~{N}-[4-(6,7-dimethoxyquinazolin-4-yl)oxyphenyl]-2-(1-ethylpyrazol-4-yl)ethanamide | C23 H23 N5 O4 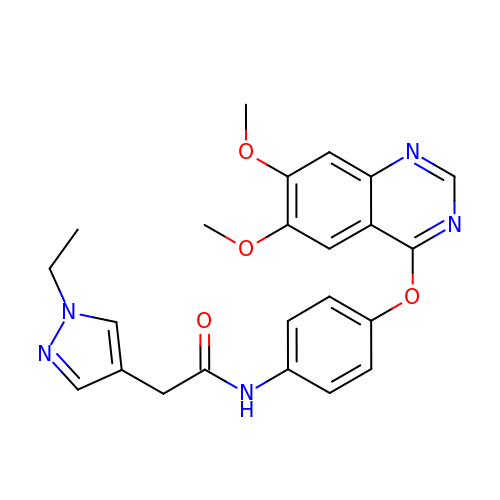| LQRLWWAVCUCERB-UHFFFAOYSA-N> GETGQLIKDTIKNTVENTVESTHSISTEATPALQAAETGATSNASDESMIETRNVVNTHGVAETSLEGFYGRAGLVAMFTTEGGIRSWYINFGKYVQLRAKLELLTYARFDVEFTIVAQVVDEQAKVKDFNVDYQVMYVPPGASAPDGQDSFQWQSSCNPSVISNTGLPPARVSVPFMSSANAYSFSYDGYIQFGDTSSSSYGILPIHYLGQLVVRTCEDLDSARLRVRIYAKPKHMRGWIPRSPRMRPYVSRFTGIYTDAPSFCVNRESITTAG;> SAEACGYSDRVAQLTLGNSTIT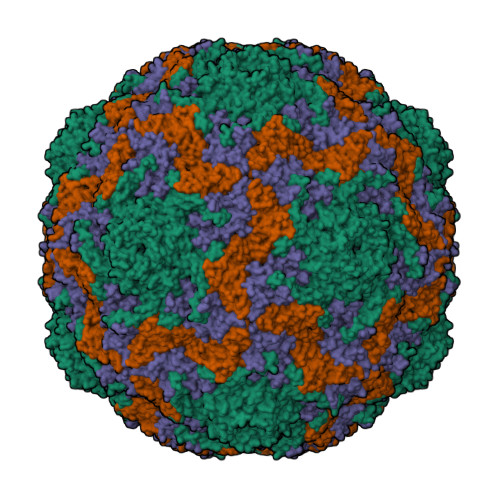TQEAANIVVAYGRWPSGLRDTDATAVDKPTQPGVSAERFYTLPSVQWTTSFTGHYWKLPDALSDLGLFGQNLQFHYLYRGGWAIHVQCNATKFHQGTLLVVAVPEHKIQAQSNPSFGRTNPGEAGAACQFPFTFEDGTALGNALIYPHQWINLRTNNSATLVLPYVNAIPMDSGIKHNNWTLLVIPIVPLEYAVGATTFVPITVTIAPMCTEYNGLRAAVTQ;> GCPTLYTPGSGQFLTTDDFQTPCMLPKFQPTPVIDIPGEVKNFLEVIQVESLVEINNVSGVEGVARYRIPLNVQDAMDGQIMAVRVDPGADGPMQSTLLGVFTRYYTQWSGSLDFTFMFCGTFMTTGKVIIAYTPPGGDQPGSRQQAMLGTHVVWDFGLQSSITLVVPWISSGHFRGTSLDNTIYKYRYYEAGYITMWYQTNMVVPPNFPTEASILMFVAAQPNFSLRILKDRPDITQVASLQ;> MGAQLSKNTAGSHTTGTYATGGSSIHYTNINYYENAASNSLNKQDFTQDPDKFTRPVADIMKEAAVPLKSP>[2x]GIDTIIEQMRKKTMKTGFDFNIMVVGQSGLGKSTLVNTLFKSQVSRKASSWNREEKIPKTVEIKAIGHVIEEGGVKMKLTVIDTPGFGDQINNENCWEPIEKYINEQYEKFLKEEVNIARKKRIPDTRVHCCLYFISPTGHSLRPLDLEFMKHLSKVVNIIPVIAKADT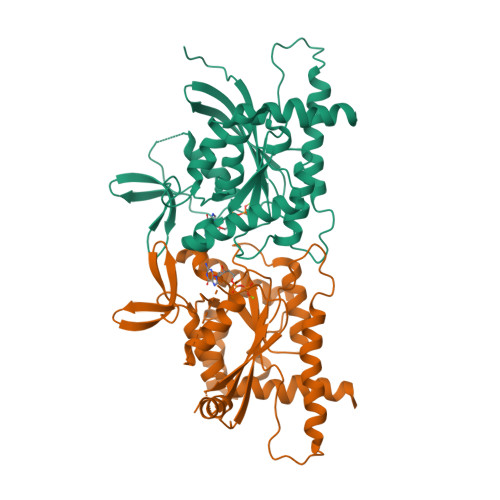MTLEEKSEFKQRVRKELEVNGIEFYPQKEFDEDLEDKTENDKIRQESMPFAVVGSDKEYQVNGKRVLGRKTPWGIIEVENLNHCEFALLRDFVIRTHLQDLKEVTHNIHYETYRAKRL>[2x]GSHMMGNKQTVFTHE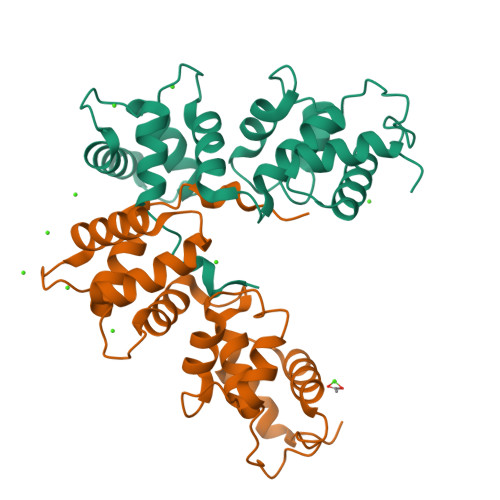QLEAYQDCTFFTRKEIMRLFYRYQDLAPQLVPLDYTTCPDVKVPYELIGSMPELKDNPFRQRIAQVFSEDGDGHMTLDNFLDMFSVMSEMAPRDLKAYYAFKIYDFNNDDYICAWDLEQTVTKLTRGELSAEEVSLVCQHVLDEADGDHDGRLSLEDFQNMILRAPDFLSTFHIRI6-chloro-3-[1-(4-chlorobenzyl)-4-phenyl-1H-imidazol-5-yl]-1H-indole-2-carboxylic 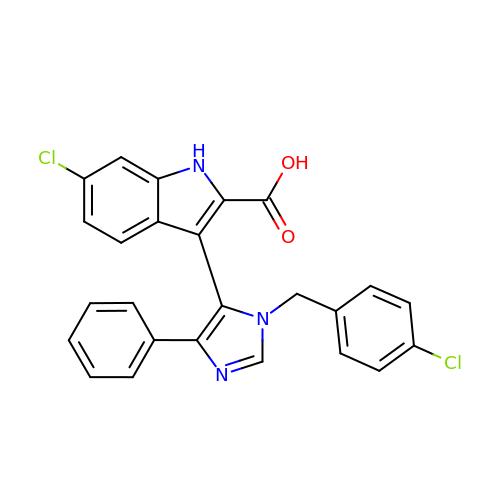acid | C25 H17 Cl2 N3 O2 | QZJRNGXHRQJBJH-UHFFFAOYSA-N> HHHHHHATGDDHFYAEYLMPGLQRLLDPESAHRLAVRVTSLGLLPRATFQDSDMLEVKVLGHKFRNPVGIAAGFDKNGEAVDGLYKLGFGFVEVGSVTPQPQEGNPRPRVFRLPEDQAVINRYGFNSHGLSVVEHRLRARQQKQAQL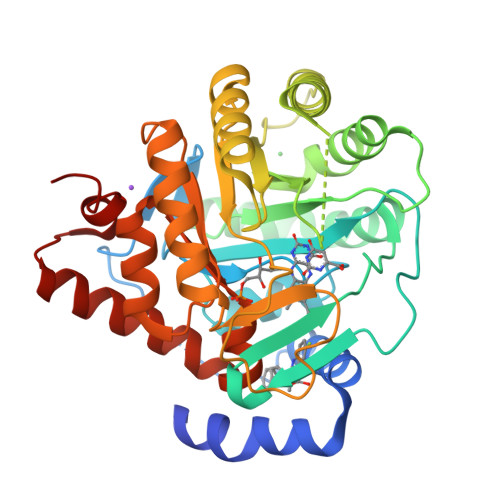TADGLPLGINLGKNKTSEDAAADYAEGVRTLGPLADYLVVNVSSPNTAGLRSLQGKTELRHLLSKVLQERDALKGTRKPAVLVKIAPDLTAQDKEDIASVARELGIDGLIVTNTTVSRPVGLQGALRSETGGLSGKPLRDLSTQTIREMYALTQGRIPIIGVGGVSSGQDALEKIQAGASLVQLYTALIFLGPPVVVRVKRELEALLKERGFTTVTDAIGADHRR> ADDEKNALPISKDGYIRVPKERVNVNLTSIKKLREKVDDSIHRELTDIFANLNYVGVVDEERRLAAIQHDLKLFLIDYGSVCYELFYQIGLTDFANFGKINLQSTNVSDDIVLYNLLSEFDELNDDASKEKI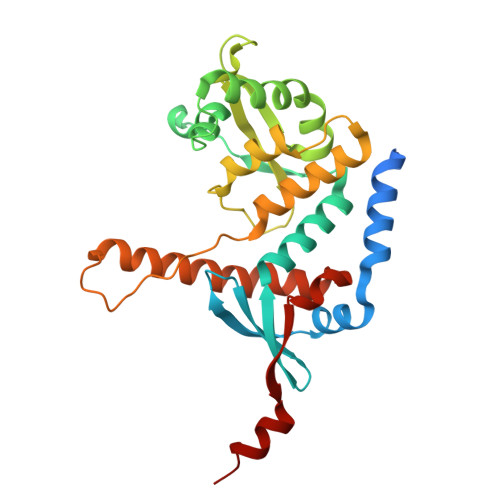ISKIWDMSSMLNEYYSIELVNDGLDNDLKSVKLKSLPLLLKGYIPSLVKLPFFIYRLGKEVDWEDEQECLDGILREIALLYIPDMVPKVDTSDASLSEDEKAQFINRKEHISSLLEHVLFPCIKRRFLAPRHILKDVVEIANLPDLYKVFERC>[3x]MKMASNDAAPSTDGAAGLVPESNNEVMALEPVAGAALAAPVTGQTNIIDPWIRANFVQAPNGEFTVSPRNAPGEVLLNLELGPELNPYLAHLARMYNGYAGGMEVQVMLAGNAFTAGKLVFAAVPPHFPVENLSPQQITMFPHVIIDVRTLEPVLLPLPDVRNNFFHYNQKDDPKMRIVAMLYTPLRSNGSGDDVFTVSCRVLTRPSPDFDFTYLVPPTVESKTKPFTLPILTL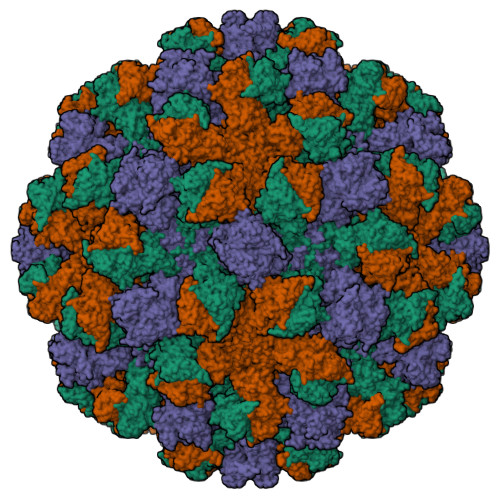GELSNSRFPVSIDQMYTSPNEVISVQCQNGRCTLDGELQGTTQLQVSGICAFKGEVTAHLQDNDHLYNITITNLNGSPFDPSEDIPAPLGVPDFQGRVFGVITQRDKQNAAGQSQPANRGHDAVVPTYTAQYTPKLGQVQIGTWQTDDLKVNQPVKFTPVGLNDTEHFNQWVVPRYAGALNLNTNLAPSVAPVFPGERLLFFRSYLPLKGGYGNPAIDCLLPQEWVQHFYQEAAPSMSEVALVRYINPDTGRALFEAKLHRAGFMTVSSNTSAPVVVPANGYFRFDSWVNQFYSLAPMGTGNGRRRIQ N-{3-[(1R,5S,6R)-3-amino-5-methyl-2-oxa-4-azabicyclo[4.1.0]hept-3-en-5-yl]-4-fluorophenyl}-5-methoxypyrazine-2-carboxamide | C18 H18 F N5 O3 | 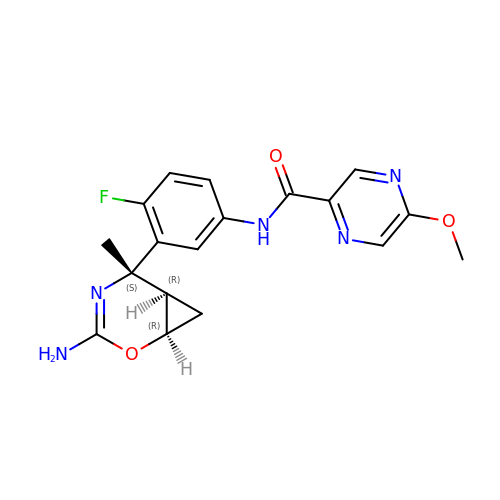LUOFRFUNXXGHFC-UCMVZMLTSA-N> STNDNIKDLLDWYSSGSDTFTNSEVLDNSLGSMRIKNTDGSISLIIFPSPYYSPAFTKGEKVDLNTKRIKKSQ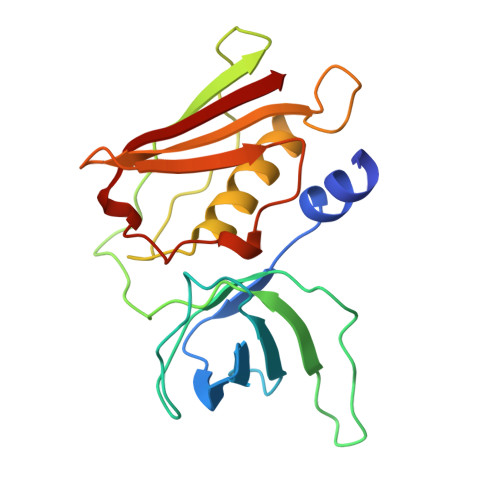HTSEGTWIHFQISGVTNTEKLPTPIELPLKVKVHGKDSPLKYWPKFDKKQLAISTLDFKIRHQLTQTHGLYRSSDKTGGYWKITMNDGSTYQSDLSKKFEYNTEKPPINIDEIKTIEAEIN> SGSFELRLKYFSNDHGRDNEGRCCSGESDGATGKCLGSCKTRFRVCLKHYQATIDTTSQCTYGDVITPILGENSVNLTDAQRFQNKGFTNPIQFPFSFSWPGTFSLIVEAWHDTNNSGNARTNKLLIQRLLVQQVLEVSSEWKTNKSESQYTSLEYDFRVTCDLNYYGSGCAKFCRPRDDSFGHSTCSETGEIICLTGWQGDYCHIPKCAKGCEHGHCDKPNQCVCQLGWKGALCN

The Notch signalling pathway is highly conserved and plays key roles in many aspects of development and homeostasis. Canonical Notch signalling involves a simple cascade, whereby ligand binding induces successive cleavages to release the Notch intracellular domain (NICD) which translocates to the nucleus and directly regulates gene expression with its binding partners (Kovall, 2008; Kovall & Blacklow, 2010; Bray, 2016; Kovall et al, 2017). All Notch ligands have a similar architecture, with an extracellular domain consisting of multiple (7, 8, or 16) epidermal growth factor (EGF) repeats, a so‐called Delta/Serrate/Lag‐2 (DSL) domain and a highly conserved N‐terminal region (Bray, 2006; D’Souza et al, 2008; Kopan & Ilagan, 2009; Kovall & Blacklow, 2010). Receptor binding involves the N‐terminal portion including the DSL and N‐terminal domains (Cordle et al, 2008; Luca et al, 2015, 2017).

To determine whether the Drosophila ligands adopt the same arrangement as their mammalian counterparts, we solved the structures of the N‐terminal region of Drosophila Delta and Serrate as well as the ligand‐binding region of Drosophila Notch (EGF11‐13; Fig EV1A–E). Notable exceptions to the overall conserved arrangements are the β1‐2 and β5‐6 loops which exhibit different lengths and folding in the ligands. These highly variable loops protrude apically from the C2 domain core and are positioned far from the Notch‐binding interface. The β1‐2 loop (blue for Delta, at top) adopts a different conformation in Delta than in Serrate despite conservation of the two stabilizing disulphides; (E) Notch—one copy of EGF11‐13. C Isolated structure of N‐terminal Delta, with residues deleted in ∆β1‐2 highlighted as red Van Der Waals spheres. Purified N‐terminal fragments (NE3 variants) were therefore used to test the liposome‐binding capability of variants in which 5 amino acids were deleted from the β1‐2 loop, hereafter referred to as DeltaΔβ1‐2. Using a liposome composition of phosphatidylcholine (PC): phosphatidylserine (PS): phosphatidylethanolamine‐fluoroscein (PE) (80:15:5), we could detect binding of wild‐type Delta (DeltaWT) fragment to the liposomes as seen for mammalian Notch ligands. This binding was compromised when the variable β1‐2 loop was shortened, resulting in the deletion of residues GATGK; DeltaΔβ1‐2 fragment exhibited a significant reduction in binding when compared to that from DeltaWT. In comparison, the variant with the loop deletion, the DeltaΔβ1‐2 fragment, retained Notch binding as predicted from the fact that the loop is positioned far away from the Notch‐binding interface. A deletion mutation affecting one of these, a loop between the β1 and β2 strands of the C2 domain core, was sufficient to compromise liposome binding.> PAGPEIRRAADNLEAAIKGKPLTDVWFAFPQLKTYQSQLIGQHVTHVETRGKALLTHFSNDLTLYSHNQLYGVWRVVDTGEEPQTTRVLRVKLQTADKTILLYSASDIEMLRPEQLTTHPFLQRVGPDVLDPNLTPEVVKERLLSPRFRNRQFAGLLLDQAFLAGLGNYLRVEILWQVGLTGNHKAKDLNAAQLDALAHALLEIPRFSYATRGQVDENKHHGALFRFKVFHRDGEPCERCGSIIEKTTLSSRP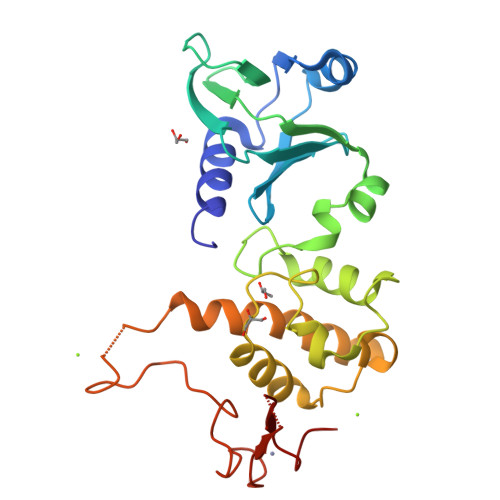FYWCPGCQH> QEDFPPRIVEHPSDLIVSKGEPATLNCKAEGRPTPTIEWYKGGERVETDKDDPRSHRMLLPSGSLFFLRIVHGRKSRPDEGVYVCVARNYLGEAVSHNASLEVAILRDDFRQNPSDVMVAVGEPAVMECQPPRGHPEPTISWKKDGSPLDDKDERITIRGGKLMITYTRKSDAGKYVCVGTNMVGERESEVAELTVLERPSFVKRPSNLAVTVDDSAEFKCEARGDPVPTVRWRKDDGELPKSRYEIRDDHTLKIRKVTAGDMGSYTCVAENMVGKAEASATLTVQEPPHFVVKPRDQVVALGRTVTFQCEATGNPQPAIFWRREGSQNLLFSYQPPQSSSRFSVSQTGDLTITNVQ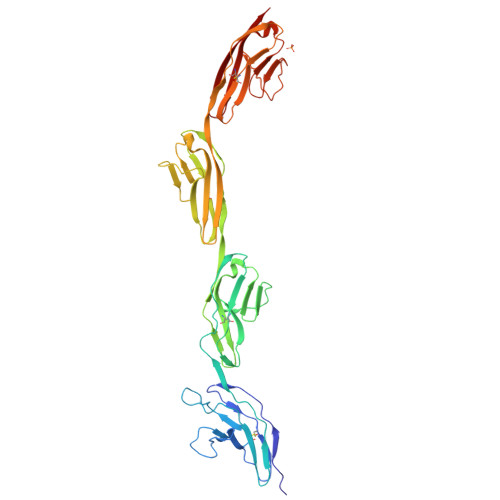RSDVGYYICQTLNVAGSIITKAYLEVTD5-[2-(piperidin-4-yl)-1,3-thiazol-5-yl]-3-[(pyridin-4-yl)methoxy]pyridin-2-amine | C19 H21 N5 O S | 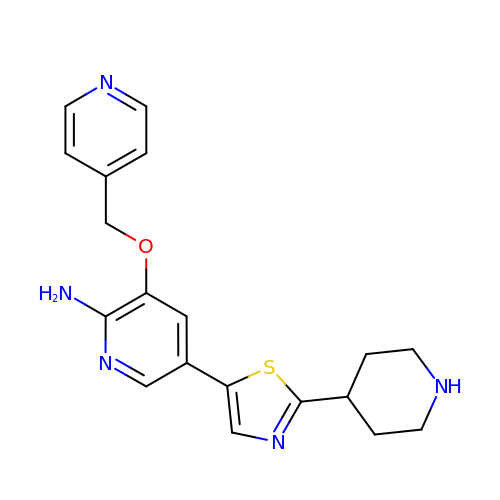HSEGDFMLRPWOHH-UHFFFAOYSA-N> KVFEVHVRPKKLAVEPKGSLEVNCSTT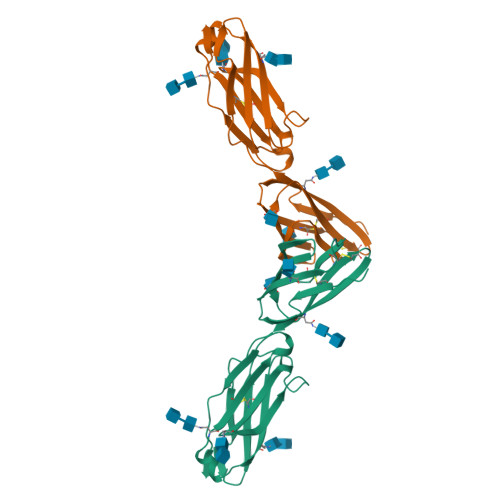CNQPEVGGLETSLNKILLDEQAQWKHYLVSNISHDTVLQCHFTCSGKQESMNSNVSVYQPPRQVILTLQPTLVAVGKSFTIECRVPTVEPLDSLTLFLFRGNETLHYETFGKAAPAPQEATATFNSTADREDGHRNFSCLAVLDLMSRGGNIFHKHSAPKMLEIY> IRVFDVWKKYKYYKKPQDRLKEIIFRKPFHEELWVLKGINLEIEKGEVLGIVGPNGAGKSTLLKVITGVTEPDKGFVERSGKVVGLLELGTGFNYELSGLENIYVNASLLGLSRREIDEKLESIIEFSELDDFINKPLKTYSSGMIMRLAFSIAIHTEPECFIIDEALAVGDAHFQQKCFRKLKEHKQKGGSIIFVSHDM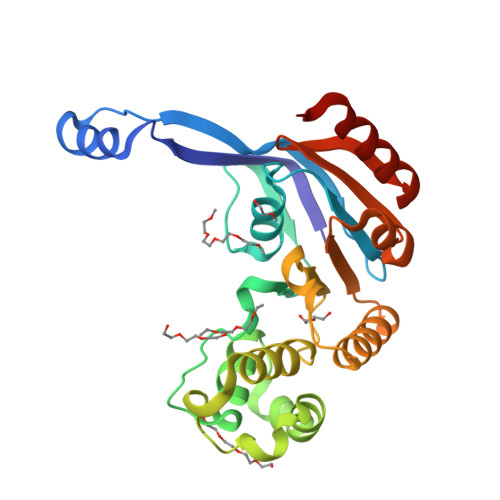NAVKILCDRAILLHKGEIIEEGSPETVTQAYYKLKLHHHHHH> SMSSFEGQMAEYPTISIDRFDRENLRARAYFLSHCHKDHMKGLRAPTLKRRLECSLKVYLYCSPVTKELLLTSPKYRFWKKRIISIEIETPTQISLVDEASGEKEEIVVTLLPAGHCPGSVMFLFQGNNGTVLYTGDFRLAQGEAARMELLHSGGRVKDIQSVYLDTTFCDPRFYQIPSREECLSGVLELVRSWITRSPYHVVWLNCKAAYGYEYLFTNLSEELGVQVHVNKLDMFRNMPEILHHLTTDRNTQIHACRHPKAEEYFQWSKLPCGITSRNRIPLHIISIKPSTMWFGERSRKTNVIVRTGESSYRACFSFHSSYSEIKDFLSYLCPVNAYPNVIPVGTTMDKVVEILKPLCRS

Artemis (SNM1C/DCLRE1C) is an endonuclease that plays a key role in development of B- and T-lymphocytes and in dsDNA break repair by non-homologous end-joining (NHEJ). Artemis is phosphorylated by DNA-PKcs and acts to open DNA hairpin intermediates generated during V(D)J and class-switch recombination. Artemis belongs to a superfamily of nucleases containing metallo-β-lactamase (MBL) and β-CASP (CPSF-Artemis-SNM1-Pso2) domains. The overall fold of the catalytic core of Artemis is similar to that of SNM1A and SNM1B (2 Å backbone RMSD); it has all the key structural characteristics of human MBL fold nucleases, with the di-metal containing active site at the interface between the MBL and β-CASP domains.

We present high-resolution crystal structures of the catalytic core of Artemis (aa 1–361) containing both MBL and a β-CASP domains. The catalytic domain of Artemis (aa 3–361) fused to the basic His6-Zb tag, which confers tight binding to cation exchange columns, was produced in baculovirus-infected Sf9 cells. The protein was purified using immobilized metal affinity chromatography (IMAC) on a nickel-Sepharose column as the initial step. We compared the catalytic domain purified using IMAC (which contained Ni2+ in the active site) with catalytic domain protein purified using ion exchange chromatography (avoiding IMAC), which contained predominantly Zn2+. As observed in structures of SNM1A and SNM1B, Artemis can coordinate one or two metal ions in its active site. Notably, a second metal ion binding site, unique to Artemis, with similarity to the canonical Cys2 His2 zinc-finger motif, is present in its β-CASP domain. Similar to the canonical Cys2 His2 zinc finger motif, the zinc ion coordination in Artemis’ β-CASP domain adopts a tetrahedral geometry, with coordination by two cysteine (Cys256, Cys272) and two histidine (His228, His254) residues. However, in the case of Artemis the metal ion coordination site is sandwiched between two β-sheets instead of an α-helix and two antiparallel β-sheets. Neither the presence of copurifying Ni ion in the active site, nor the truncation of the C-terminal tail, appear to substantially inhibit the activity of Artemis. Thus, using radio-labelled gel-based nuclease assays, we showed that the truncated Artemis catalytic domain (aa 1–361) with either copurifying Zn or Ni ions (as observed crystallographically in the same preparations) have similar activity with the full-length Artemis construct (aa 1–693).> GQLAPGITMSEIDRIAQNIIKSHLETCQYTMEELHQLAWQTHTYEEIKAYQSKSREALWQQCAIQITHAIQYVVEFAKRITGFMELCQNDQILLLKSGCLEVVLVRMCRAFNPLNNTVLFEGKYGGMQMFKALGSDDLVNEAFDFAKNLCSLQLT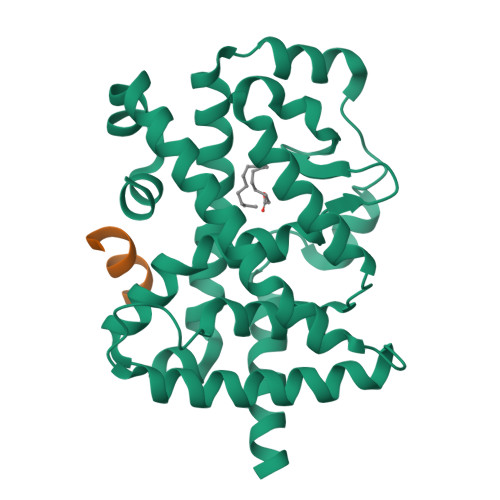EEEIALFSSAVLISPDRAWLLEPRKVQKLQEKIYFALQHVIQKNHLDDETLAKLIAKIPTITAVCNLHGEKLQVFKQSHPDIVNTLFPPLYKELFNP;> RHKILHRLLQEGSPS>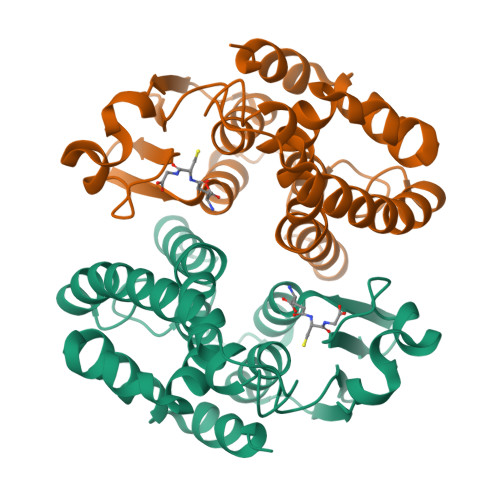 MAPVKVFGPAMSTNVARVTLCLEEVGAEYEVVNIDFNTMEHKSPEHLARNPFGQIPAFQDGDLLLWESRAISKYVLRKYKTDEVDLLRESNLEEAAMVDVWTEVDAHTYNPALSPIVSQCLFNPMMRGLPTDEKVVAESLEKLKKVLEVYEARLSKHSYLAGDFVSFADLNHFPYTFYFMATPHAALFDSYPHVKAWWDRLMARPAVKKIAATMVPPKA> GSHFYFLSKRRRNLLRNPAGEEDLEGWSDVEHGGDGWKVEELPGDNGVEFTQDDSVKKYFASSFEWCRKAQVIDLQAEGYWEELLDTTQPAIVVKDWYSGRTDAGSLYELTVRLLSENEDVLAEFATGQVAVPEDGSWMEISHTFIDYGPGVRFVRFEHGGQDSVYWKGWFGARVTNSSVWVE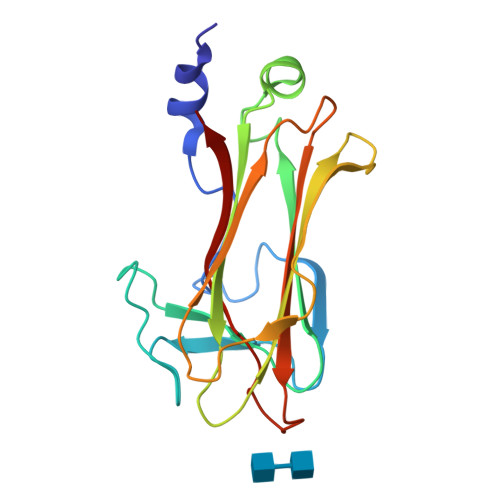P>[4x]HMLGKIALEEAFALPRFEEKTRWWASLFSTDAETHVKEITDINKIRIEHADKHGVGYQILSYTSPGVQDIWDPVEAQALAVEINDYIAEQVRVNPDRFGAFATLSMHNPKEAADELRRCVEKYGFKGALVNDTQRAGPDGDDMIFYDNADWDIFWQTCTELDVPFYMHPRNPTGTIYEKLWADRKWLVGPPLSFAHGVS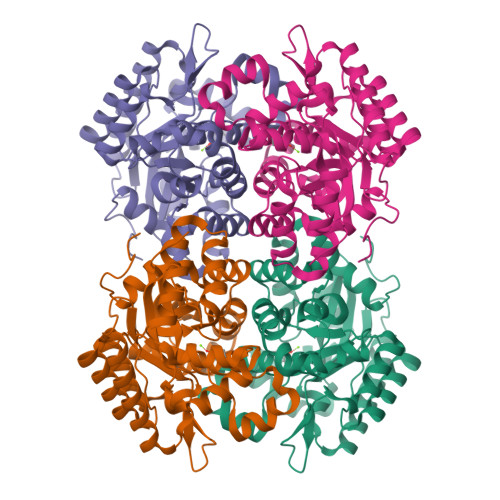LHVLGMVTNGVFDRHPKLQIIMGHLGEHVPFDMWRINHWFEDRKKLLGLAETCKKTIRDYFAENIWITTSGHFSTTTLNFCMAEVGSDRILFSIDYPFETFSDACEWFDNAELNGTDRLKIGRENAKKLFKLDSYKDSSA>MSKNHQKVVLVGDGAVGSSYAFAMAQQGIAEEFAIVDIIKERTEGDAMDLEDATAFTAPKNIYSADYDTCKDADLVVITAGAPQKPGETRLQLVDKNLKIIKSVVEPIVKSGFDGIFLVAANPVDILTYAVQKLSGFPKNKVVGSGTSLDSARLRVALGKKLDVDPRDVIANIMGEHGDSEFAAYSSATVGGKPLLDIAKDEGISEDELLKIEDDVRNKAYEIINRKGATFYGVATALMRISKAILRDENSVLPIGAPMNGEYGLNDLYIG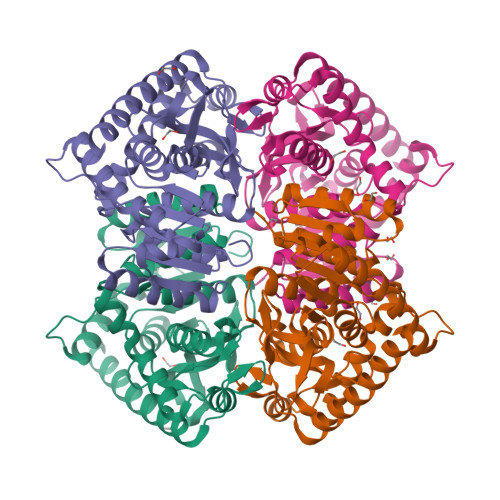TPAVVNASGVAKVIEVPLNDREKKAMADSAKQLEEVAKNGMAKLQGNN[2x]N-cyclohexyl-4-imidazo[1,2-a]pyridin-3-yl-N-methylpyrimidin-2-amine | C18 H21 N5 | 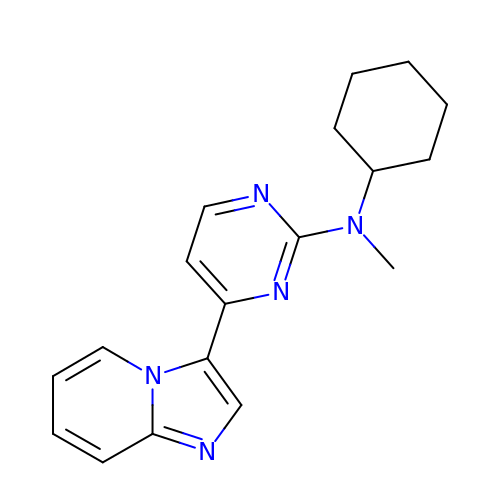HYNNWLVWJXWXFO-UHFFFAOYSA-N>MVLPNFKENLEKYAKLLVANGINVQPGHTLALSIDVEQRELAHLIVKEAYALGAHEVIVQWTDDVINREKFLHAPMERLDNVPEYKIAEMNYLLENKASRLGVRSSDPGALNGVDADKLSASAKAMGLAMKPMRIATQSNKVSWTVAAAAGLEWAKKVFPNAASDEEAVDFLWDQIFKTCRVYEADPVKAWEEHAAILKSKADMLNKEQFSALHYTAPGTDLTLGLPKNHVWESAGAVNAQGEEFLPNMPTEEVFT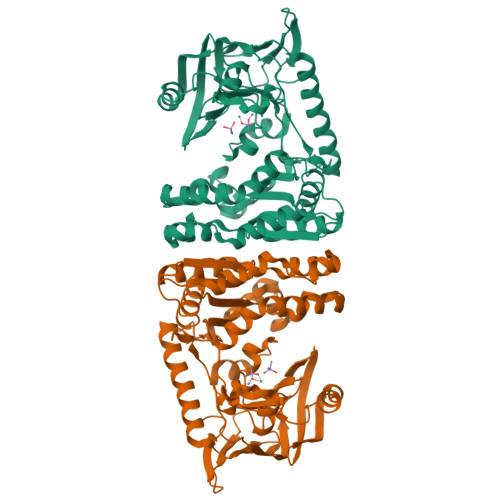APDFRRADGYVTSTKPLSYNGNIIEGIKVTFKDGQIVDITAEKGDQVMKDLVFENAGARALGECALVPDPSPISQSGITFFNTLFDDNASNHLAIGAAYATSVVDGAEMSEEELEAAGLNRSDVHVDFMIGSNQMDIDGIREDGTRVPLFRNGNWAN[2x]>MGHHHHHHTQILIVEDEQNLARFLELELTHENYNVDTEYDGQDGLDKALSHYYDLIILDLMLPSINGLEICRKIRQQQSTPIIIITAKSDTYDKVAGLDYGADDYIVKPFDIEELLARIRAILRRQ[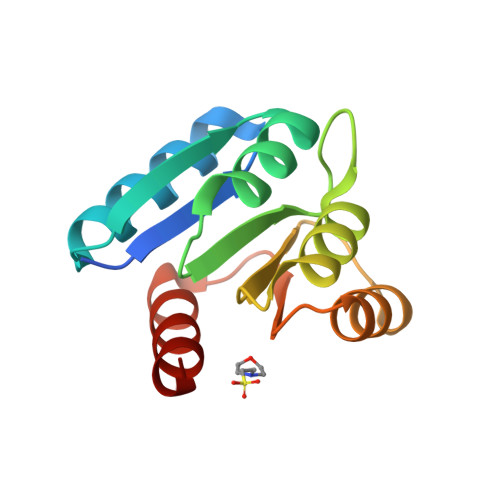2x]>[4x]MIRTFETHKIRKTAELSSALWNFHTIGTQGEEAVIQAPVPGCWENYPDTVSYRGQASYSREFEAKGNIRLEFKGVSHTASVLVDGKPVGSHYNAYTPFDVVLKDIRPGIHQLEVIADNSFGPDSALHVPNDYQSYGGISRGVVLEELGEAYLSWIHFTPFLRKDGWYGKAEICVRNLSSGRLDGSVEVEIGKNSFAVLPIVLEGEEEKSFSTEELPCPWAECWSPESPVLYLITAVLR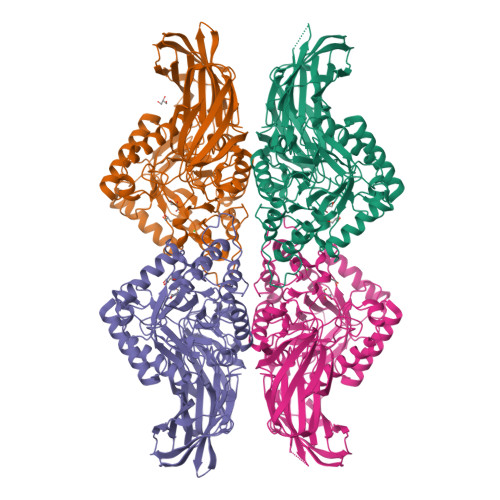TADGAADDIIDRVGFREIRTEGKDILLNGRKLRIKGFCRHEDHPQFGCALPFSAMQHDLMLIKDLGANSIRTVHYPNDELFLDLCDEQGILVWEENHARGLSEENMRNPHFKQQCGDCIREMITAHYNHPSIYIWGILNECASDTEYGRECYSEQYELIKSLDPYRPRSSASCRFKTDICLGYPEVVSYNIYPKWYHDVPVEDYLDELYQWIQNESEGTGKPFLITEIGAGAIYGYRTPAHVKWSEEYQVQALKEQLQAVFSREGCSGVYIWQFCDVRVCDSWFGSRPRTMNNKGIVDEYRRPKLAYEVVKDSYRSLGNYFENLYFQSGSHHHHHH>GSQKERLLDELTLEGVARYMQSERCRRVICLVGAGISTSAGIPDFRSPSTGLYDNLEKYHLPYPEAIFEISYFKKHPEPFFALAKELYPGQFKPTICHYFMRLLKDKGLLLRCYTQNIDTLERIAGLEQEDLVEAHGTFYTSHCVSASCRHEYPLSWMKEKIFSEV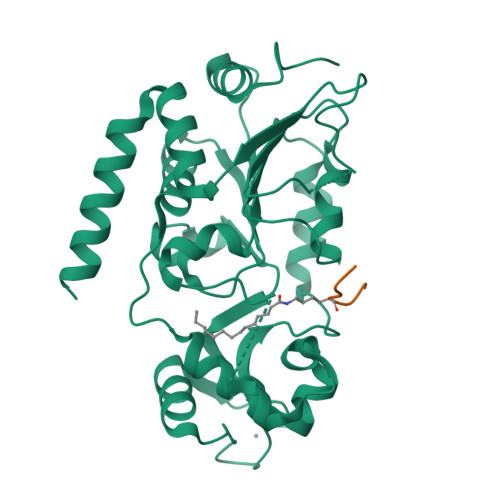TPKCEDCQSLVKPDIVFFGESLPARFFSCMQSDFLKVDLLLVMGTSLQVQPFASLISKAPLSTPRLLINKEKAGGGGMDFDSKKAYRDVAWLGECDQGCLALAELLGWKKELEDLVRREHASIDAQS[2x];>TARXSTG[2x]> MWRP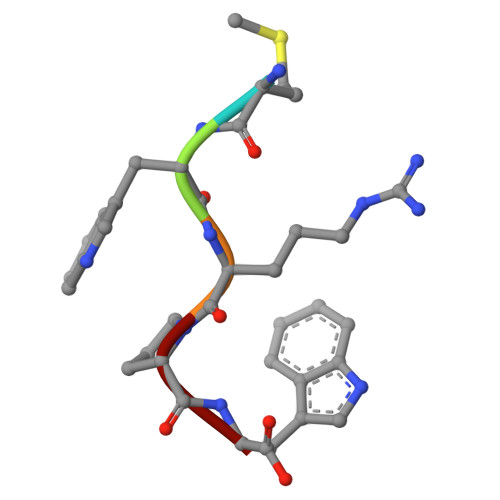W> MHHHHHHSSGRENLYFQGEKEDHLKTIVKKHLSPENFDPTNRKYWVYDDHLKNFVNFKFTGDVRPWPLSKINHVPSHIERPDYAISSIPESELIYKRKSDIYVNNEEEIQRIREACILGRKTLDYAHTLVSPGVTTDEIDRKVHEFIIKNNAYPSTLNYYKFPKSCCTSVNEIVCHGIPDYRPLKSGDIINIDISVFYKGVHSDLNETYFVGDINDVPKEGKELVETCYFSLMEAIKKCKPGMFYKNIGTLIDAYVSKKNFSVVRSYSGHGVGKLFHSNPTVPHFKKNKAVGIMKPG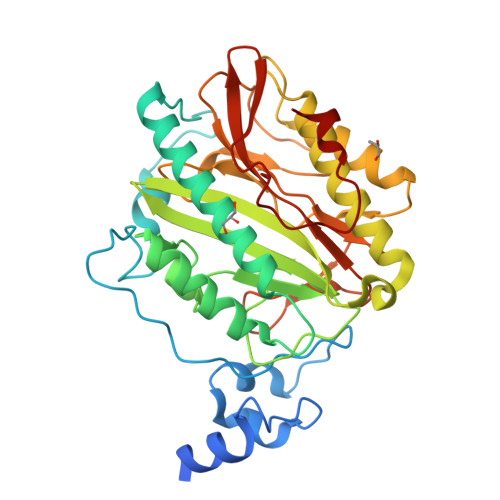HVFTIEPMINQGHYSDVLWPDQWTSATSDGKLSAQFEHTLLITNNGVEILTKRTQDSPPLGFDTKDELYYN>XPPGPPGPPGPKGDPGPPGPPGP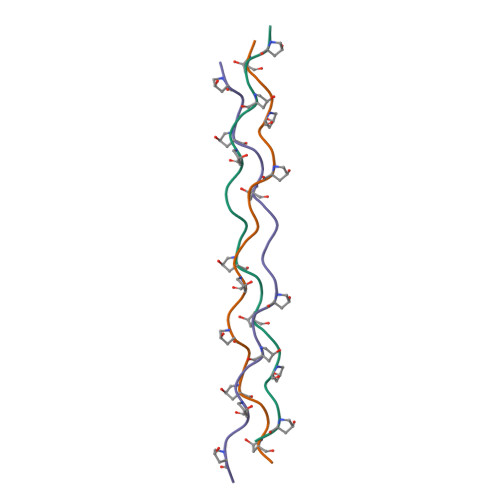PGX[6x]Type IV pili (T4P) are functionally versatile filaments widespread in prokaryotes, composed of type IV pilins and assembled by conserved multiprotein machineries. We show that PilB is a modular pilin with a bulky module “grafted” onto a small pilin module, which directly mediates adhesion of S. sanguinis to host cells/proteins. PilB, one of the three minor pilins in S. sanguinis T4P, exhibits a canonical N-terminal class III signal peptide, the defining feature of type IV pilins. The larger size of PilB is due to the presence of a C-terminal domain readily detectable by bioinformatics, which belongs to the von Willebrand factor A–like domain superfamily (InterPro entry IPR036465).

The protein readily crystallized in multiple conditions, and after optimizing the best diffracting crystals, we collected a complete dataset on crystals forming in the space group P61. The pilin module exhibits a long N-terminal α-helix packed against, not one β-sheet as usual, but two consecutive β-sheets consisting of six and three β-strands respectively, which together form the globular head of the pilin. The vWA moiety of PilB adopts a canonical vWA fold, with a central β-sheet (composed of five parallel and one antiparallel β-strands) surrounded on both sides by a series of α-helices. As in eukaryotic vWA-containing proteins, PilB exhibits a MIDAS located on top of the central β-sheet. However, in contrast to these proteins, the MIDAS in PilB is flanked by two protruding “arms,” which is reminiscent of the RrgA adhesin from Streptococcus pneumoniae. The MIDAS motif in PilB, which is formed by residues conserved in vWA-containing proteins, noncontiguous in the sequence but in close proximity in the 3D structure, is functional since it coordinates a metal ion in the crystal. We have modeled the metal as Mg+2 because of its abundance in the growth medium and the high affinity of PilB for it. The Ser206, Ser208, Thr291, and Asp319 residues in the MIDAS motif of PilB form direct hydrogen bonds with the metal through oxygen atoms, while two additional coordination sites are provided by water molecules. However, PilB can only be accommodated at the tip of the filaments because the bulky vWA module sits on top of the pilin module in the PilB structure and essentially prevents other pilin subunits from being modeled above it.

>SSRELIEREASIQAEMRTSMQYVDRTVGKATSIFILDDSKFKGSKQGLTREWSYIGLSADGKKVMNYVWNKQKQDWDVSELGTKSLYNMKLDLEFKTEGAYQDNRLISYNLTGKYPDTNNKLGIDTAISALNTKQVFSKVAKGKKGIAIAYRTDPIQGQMNIAVSFVFDTSGSMDWDLQGRNVKKTGNESRMDILRKKSVIMIKDLAEIGNISVNLVGFSTSAKYIQQNFSNLDNGTNTIIATITKRENLNPDGVTNPGDGLRYGMISLQSQPAQLKYIVLLTDGIPNAYLVDSRALYAGNRVDLSQGAGRVTFNNPIYDLSPTLGYEYSRLGYDLYSRDSITRENSIAYAGEVSKKFGLGIKRVNVIGFSGVNHEIAYGQSLTDRIGEGGMETKYVSATNEEALQKTFSDIKKQIQQDLWFVSGP[2x]>[4x]MASQPNSSAKKKEEKGKNIQVVVRCRPFNLAERKASAHSIVECDPVRKEVSVRTGGLADKSSRKTYTFDMVFGASTKQIDVYRSVVCPILDEVIMGYNCTIFAYGQTGTGKTFTMEGERSPNEEYTWEEDPLAGIIPRTLHQIFEKLTDNGTEFSVKVSLLEIYNEELFDLLNPSSDVSERLQMFDDPRNKRGVIIKGLEE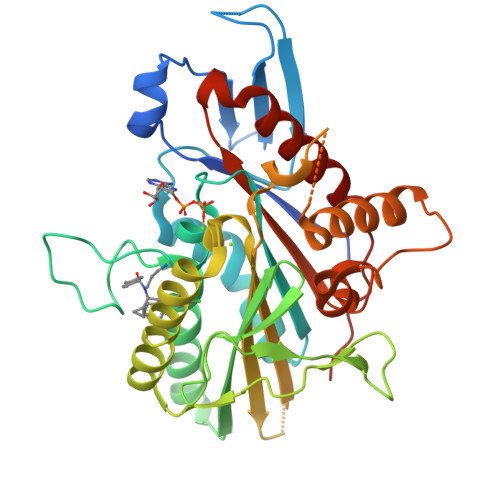ITVHNKDEVYQILEKGAAKRTTAATLMNAYSSRSHSVFSVTIHMKETTIDGEELVKIGKLNLVDLAGSENIGRSGAVDKRAREAGNINQSLLTLGRVITALVERTPHVPYRESKLTRILQDSLGGRTRTSIIATISPASLNLEETLSTLEYAHRAKNILNKPEVNQK>[2x]MEKRMSTQQRAAGNACPTAAFSFDPARLAQRRRWAGAFAALCGLALSPSALLAEEHSQHQDHAVELAPSVVTGVAQSSPLTIVTNPKEPRQPVPASDGADYLKTIPGFAVIRNGGSNGDPVLRGMFGSRLNILTNGGMMLGACPNRMDAPTSYISPETYDKLTVIKGPQTVLWGPGASAGTILFEREPERFGELGSRVNASLLAGSNGRFDKVLDAAAGNRLGYLRFTGNHAQSDDYEDGAGNTVPSRWKKWNGDVAVGWTPDEDTLIELTAGKGDGEARYAGRGMDGSQFKRESLGLRFVKSNVSDVLEKVEAQVYYNYADAIMDNFRLRTPDPS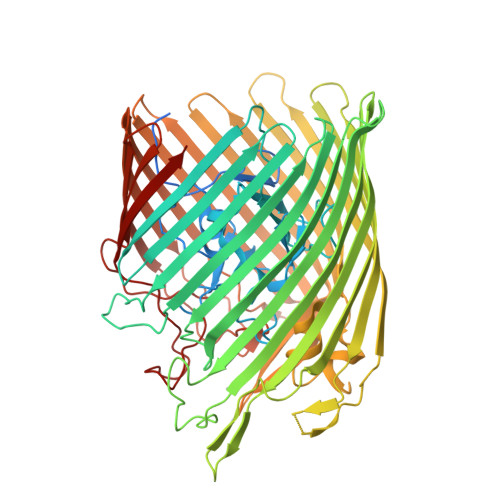SMMPMPMASQVDRRTLGGRLAATWRWDDFKLVTGVDAMRNEHRARGSKYDMMTDYYTDADQFPWSKDAVFHNYGAFGELTWFAAERDRLIGGLRLDRASVKDYRQTLKSGHMGHAMANPTANDTRADTLPSGFVRYEHDLADSPTTLYAGLGHAERFPDYWELFSPKRGPNGSVNAFDKIKPEKTTQLDFGLQYNGDKLQAWASGYVGVVQDFILFSYREGMMGSSTQATNVDARIMGGELGASYQLTGNWKTDASLAYAWGKNSSDDRALPQIPPLEARFGLTYEEGDWSAGSLWRVVAPQNRIARDQGNVVGKDFDKSAGFGVFSLNGAYRVTRNVKLSAGVDNLFDKDYTEHLNKAGDAGFGFSANETVPEPGRTFWTKVDFSF>SNAMTKIYFAGPLFSQADLRYNAYLVEQIRQLDKTIDLYLPQENAAINDKSAYADSKMIALADTENVLASDLLVALLDGPTIDAGVASEIGVAYAKGIPVVALYTDSRQQGADNHQKLDALNEIAENQFHYLNLY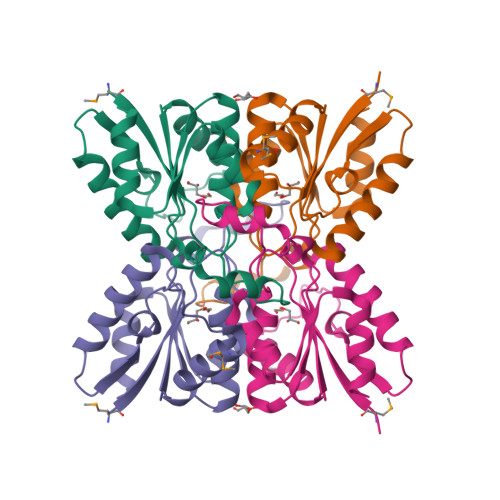TVGLIKLNGRVVSSEEDLLEEIKQRLS[2x]>[2x]MAPTSASS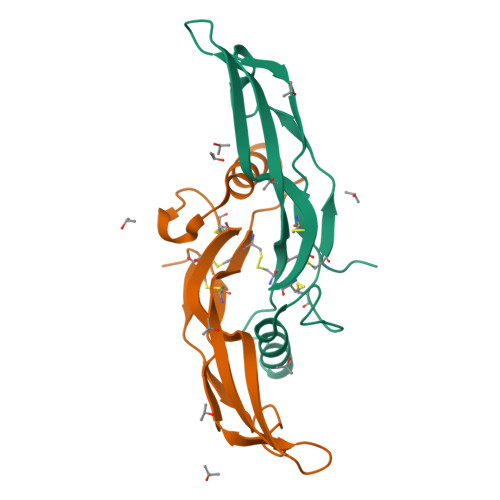RRRQQSRNRSTQSQDVARVSSASDYNSSELKTACRKHELYVSFQDLGWQDWIIAPKGYAANYCDGECSFPLNAHMNATNHAIVQTLVHLMNPEYVPKPCCAPTKLNAISVLYFDDNSNVILKKYRNMVVRACGCH> REVLTGGHSVSAPQENRIYVMDSVFMHLTESRVHVYDYTNGKFLGMVPTAFNGHVQVSNDGKKIY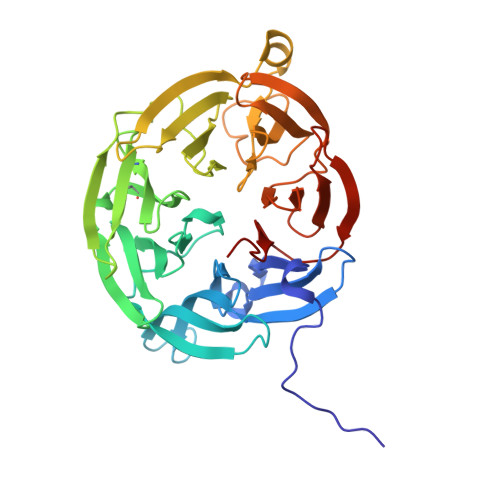TMTTYHERITRGKRSDVVEVWDADKLTFEKEISLPPKRVQGLNYDGLFRQTTDGKFIVLQNASPATSIGIVDVAKGDYVEDVTAAAGCWSVIPQPNRPRSFMTICGDGGLLTINLGEDGKVASQSRSKQMFSVADDPIFIAPALDKDKAHFVSYYGNVYSADFSGDEVKVDGPWSLLNDEDKAKNWVPGGYNLVGLHRASGRMYVFMHPDGKEGTHKFPAAEIWVMDTKTKQRVARIPGRDALSMTIDQQRNLMLTLDGGNVNVYDISQPEPKLLRTIEGAAEASLQVQFHPVGGT5'-O-[(S)-hydroxy{[(S)-hydroxy(phosphonooxy)phosphoryl]amino}phosphoryl]adenosine | C10 H17 N6 O12 P3 | 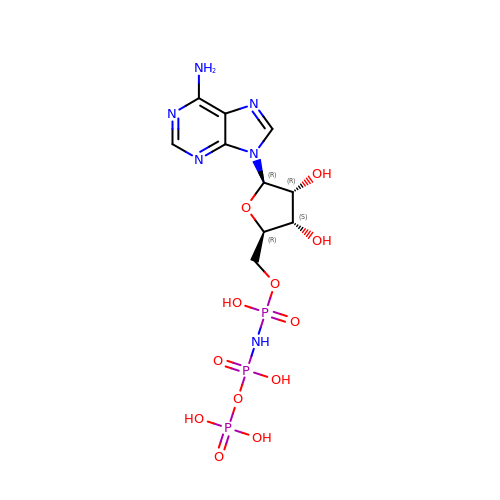WUPFAKUEHUVIDK-KQYNXXCUSA-N> ATPADWRSQSIYFLLTDRFARTDGSTTATCNTADQKYCGGTWQGIIDKLDYIQGMGFTAIWITPVTAQLPQTTAYGDAYHGYWQQDIYSLNENYGTADDLKALSSALHERGMYLMVDVVANHMGYDGAGSSVDYSVFKPFSSQDYFHPFCFIQNYEDQTQVEDCWLGDNTVSLPDLDTTKDVVKNEWYDWVGSLVSNYSIDGLRIDTVKHVQKDFWPGYNKAAGVYCIGEVLDGDPAYTCPYQNVMDGVLNYPIYYPLLNAFKSTSGSMDDLYNMINTVKSDCPDSTLLGTFVENHDNPRFASYTNDIALAKNVAAFIILNDGIPIIYAGQEQHYAGGNDPANREATWLSGYPTDSELYKLIASANAIRNYAISKDTGFVTYKNWPIYKDDTTIAMRKGTDGSQIVTILSNKGASGDSYTLSLSGAGYTAGQQLTEVIGCTTVTVGSDGNVPVPMAGGLPRVLYPTEKLAGSKICS

An innovative protein crystallization screen formulation called FUSION has been developed to help with the production of useful crystals. The concept behind the formulation of FUSION was to combine the most efficient components from the three MORPHEUS screens into a single screen using a systematic approach. Most of these additives are small molecules and ions frequently found in crystal structures of the Protein Data Bank (PDB), where they bind proteins and complexes. The efficiency of FUSION is demonstrated by obtaining high yields of diffraction-quality crystals for seven different test proteins.

In the process, two crystal forms not currently in the PDB for the proteins α-amylase and avidin were discovered.> MHLKELLEITDTTERDRSLRRAFSPYTAMIDITGSEAVALIILLNLTYRKNQVDDLLDKKLAKQALKSEDHINKCIKEIAWFHTHNLKYPDIRVSKQNLAVEPPTLHSYVLSSANYPKAYGWSHNSAKVNFAKLFVSYFKWQNQVSWLAQVLATNSDNWKSAFTSLGLSVKAFKSLCVTVKNSLPEEAIPDSVDRYSRQIRMPYHDGYLAVTPVISHVVQSKIQQAAIDKRARFSNVEFTRPAAVSMLAASLGGVINVLNYPPYIRSKYHGLSNSRAFKLNNGQTVFNVEALLKPELIKALEGIIFSNNALALKQRRQQKVKNIKELRNTLLEWFSPVFEWRLDAIENGYDLEQLESASERLEYKILSLPDNELPSLTIPLFRLLNEMLGGVSMTQRYAFHPKLMSPLKAALQWLLVNLTDQKHVLIEEDDEHYRYLHLSGIRVFDAQALSNPYCSGIPSLTAVWGMIHSYQRKLNEALGTNVRFTSFSWFIRNYSAVAGKKLPELSLQGAQQSRLKRPGIIDGKYCDLVFDLIIHIDGYEDDLQAVDSKPDILKAHFPSNFAGGVMHQPELNS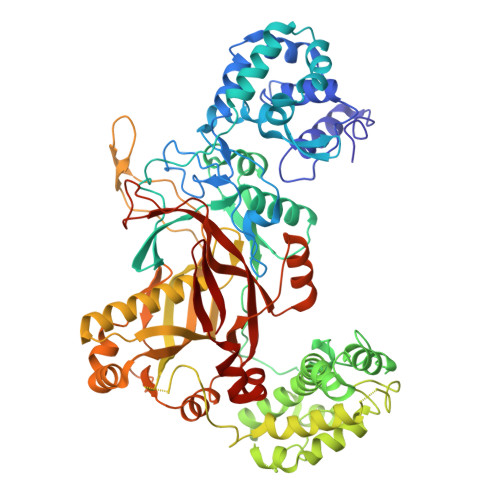NINWCCLYSNENQLFEKLRRLPLSGCWVMPTEHKIQDLDELLLLLNSDSKLSPSMMGYMLLTEPMARVGSLERLHCYAEPAIGVVKYEAATSVRLKGIGNYFNSAFWMLDAQEKFMLMKKV> MVTKTITEQRAEVRIFAGNDPAHTATGSSGISSPTPALTPLMLDEATGKLVVWDGQKAGSA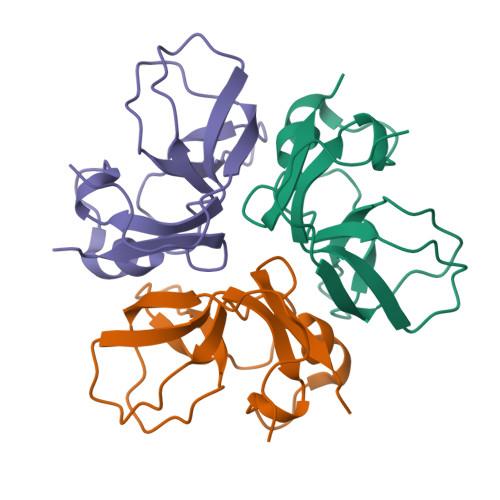VGILVLPLEGTETALTYYKSGTFATEAIHWPESVDEHKKANAFAGSALSHAALP>KPIQNQAKSVDVEYTVQFTPLNPDDDFRPGLKDTKLLKTLAIGDTITSQELLAQAQSILNKTHPGYTIYERDSSIVTHDNDIFRTILPMDQEFTYHVKNREQAYEINK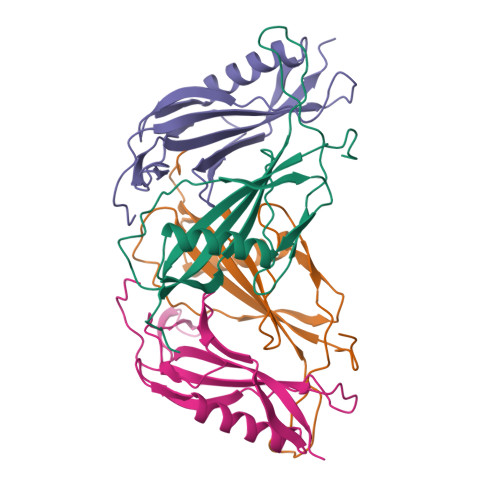KSGLNEEINNTDLISEKYYVLKKGEKPYD[4x]> KEQLASMNAIANVKATYSINGETFQIPSSDIMS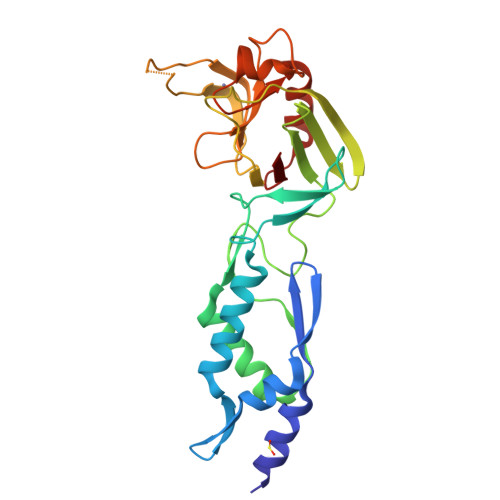WLTYNDGKVDLDTEQVRQYVTDLGTKYNTSTNDTKFKSTKRGEVTVPVGTYSWTIQTDSETEALKKAILAGQDFTRSPIVQGGTTADHPLIEDTYIEVDLENQHMWYYKDGKVALETDIVSGKPTTPTPAGVFYVWNKEEDATLKGTNDDGTPYESPVNYWMPIDWTGVGIHDSDWQPEYGGDLWKTRGSHGCINTPPSVMKELFGMVEKGTPVLVF>GMSTPTPDTDVEQVGLANTAFYEAMERGDFETLSSLWLTPADLGVDEEYHDPADAGVVSCVHPGWPVLSGRGEVLRSYALIMANTEYIQFFLTDVHVSVTGDTALVTCTENILSGGPPPDDSDELGPLVGQLVVATNVFRRTPDGWKLWSHHA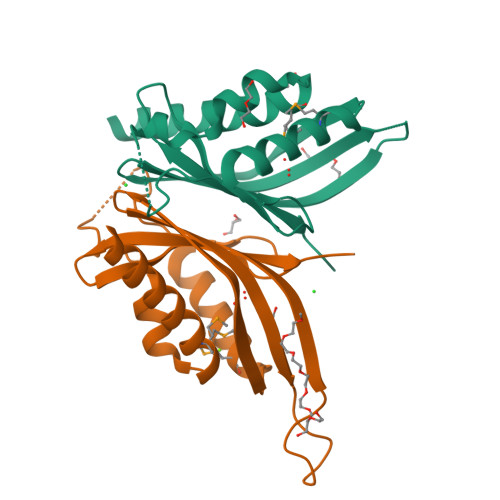SPVLAETGAEEGDESPD[3x]{(5Z)-5-[(4-methoxyphenyl)methylidene]-2,4-dioxo-1,3-thiazolidin-3-yl}acetic acid | C13 H11 N O5 S | 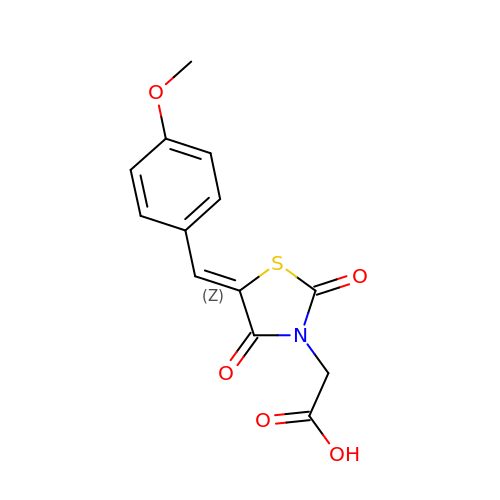VMHLNIJHJPIPKG-POHAHGRESA-N> MIYSRSKLPSEGEILIATVKQVFDYGSYVSLDEYGGLQAFLPWSEVSSKWVKNI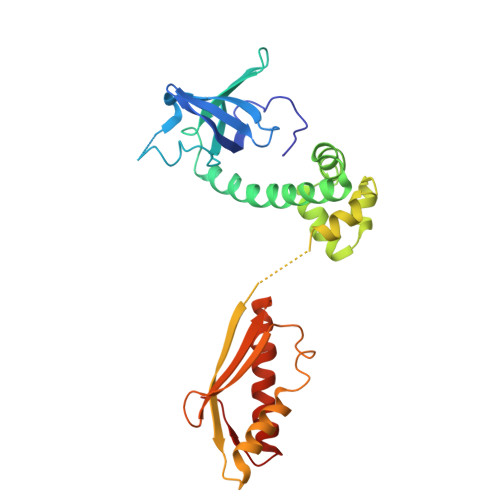RDVLKENRKVIVKVIRVDRRKGTVDVSLKKVTDDERRKKNLQWKKIQRLDKILELVSQKLKLSEKDAWEQVAWKLEAKYGDPITAIEKAVKEGEKILIDAGVPEIWVKPLLEEASKHAEERKVKMSGLITVRTNEPLGVEKIKEVISKALENIEQDYESLLNIKIYTIGAPRYRVDVVGTNPKEASEALNQIISNLIKIGKEENVDISVVKK>[2x]SDHVDLPYNLTATKIDS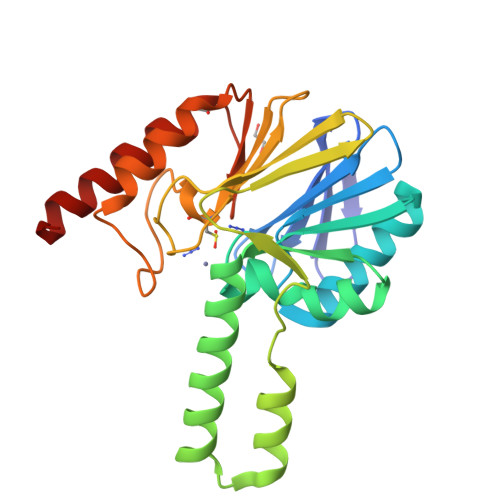DVFVVTDRDFYSSNVLVAKMLDGTVVIVSSPFENLGTQTLMDWVAKTMKPKKVVAINTHFHLDGTGGNEIYKKMGAETWSSDLTKQLRLEENKKDRIKAAEFYKNEDLKRRILSSHPVPADNVFDLKQGKVFSFSNELVEVSFPGPAHSPDNVVVYFPKKKLLFGGCMIKPKELGYLGDANVKAWPDSARRLKKFDAKIVIPGHGEWGGPEMVNKTIKVAEKAVGEMRL L-PHOSPHOLACTATE | C3 H7 O6 P | 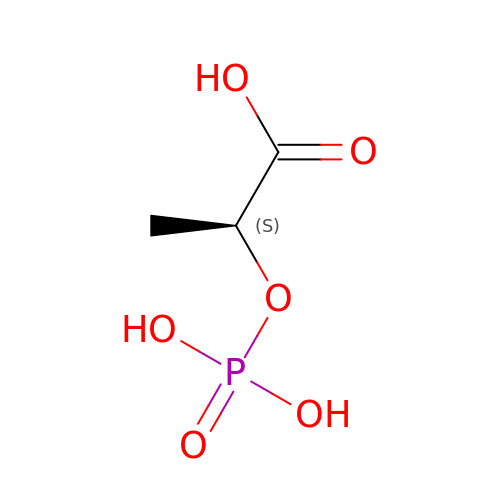CSZRNWHGZPKNKY-REOHCLBHSA-N>[2x]MPMTK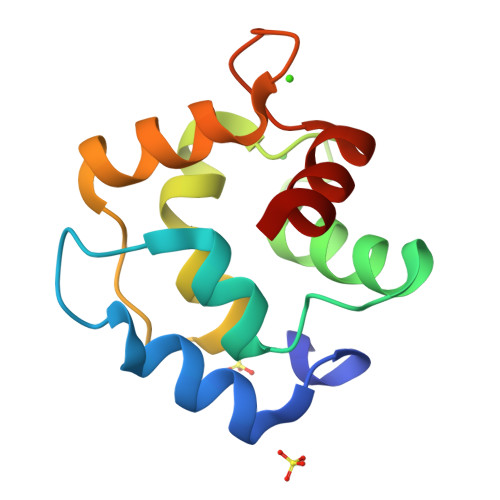VLKADDINKAVSAFKDPGTFDYKRFFQLVGLKGKSEAQVKEVFEILDKDQSGFIEEEELKSVLKGFSAHGRDLSDTETKALLAAGDSDHDGKIGADEFAKMVAQA>MEIKRRTQEERSAATREALITGARKLWGLRGYAEVGTPEIATEAGVTRGAMYHQFADKAALFRDVVEVVEQDVMARMATLVAASGAATPADAIRAAVDAWLEVSGDPEVRQLILLDAPVVLGWAGFRDVAQRYSL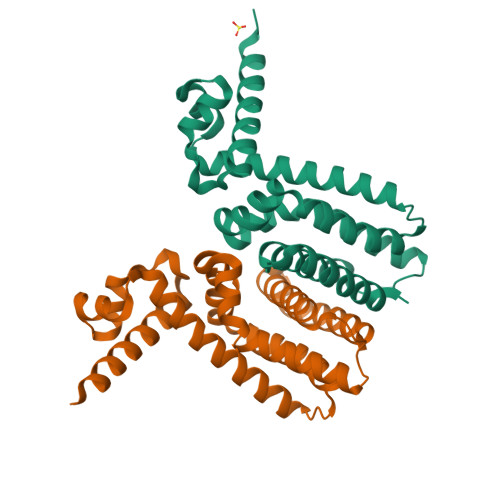GMTEQLITEAIRAGQLARQPVRPLAQVLIGALDEAAMFIATADDPKRARRETRQVLRRLIDGMLNGKLAAALEHHHHHH[4x]>MASKPQPIAAANWKCNGSQQSLSELIDLFNSTSINH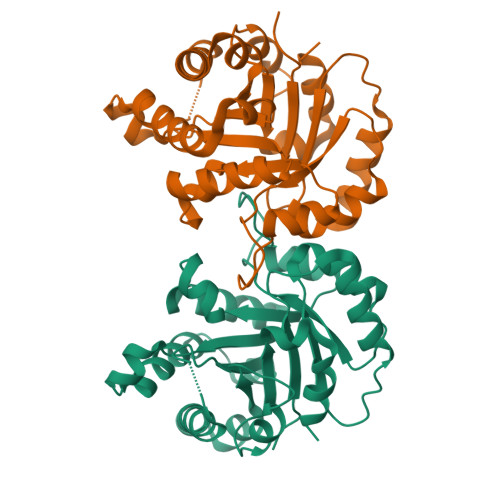DVQCVVAPTFLHIPMTKARLTNPKFQIAAQNAITRSGAFTGEVSLQILKDYGISWVVLGHSERRAYYGETNEIVADKVAAAVASGFHVIVCVGETNEEREAGRTAAVVLTQLAAVAQKLSKEAWSRVVIAYEPVWAIGTGKVATPQQAQEVHELLRRWVRSKLGTDIAAQLRILYGGSVTAKNARTLYQMRDINGFLVGGASLKPEFVEIIEATK[4x]> MPREIITLQLGQCGNQIGFEFWKQLCAEHGISPEGIVEEFATEGTDRKDVFFYQADDEHYIPRAVLLDLEPRVIHSILNSPYAKLYNPENIYLSEHGGGAGNNWASGFSQGEKIH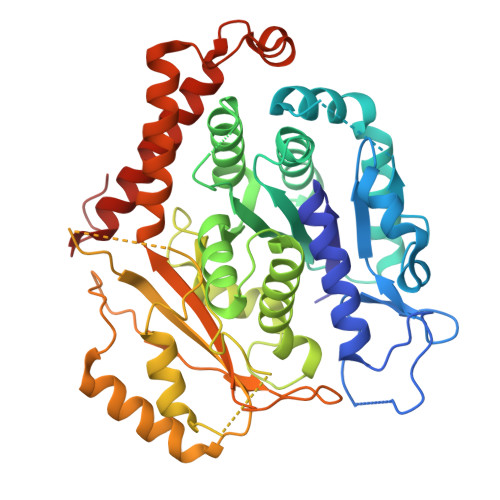EDIFDIIDREADGSDSLEGFVLCHSIAGGTGSGLGSYLLERLNDRYPKKLVQTYSVFPNQDEMSDVVVQPYNSLLTLKRLTQNADCVVVLDNTALNRIATDRLHIQNPSFSQINQLVSTIMSASTTTLRYPGYMNNDLIGLIASLIPTPRLHFLMTGYTPLTTDQSVASVRKTTVLDVMRRLLQPKNVMVSTGRDRQTNHCYIAILNIIQGEVDPTQVHKSLQRIRERKLANFIPWGPASIQVALSRKSPYLPSAHRVSGLMMANHTSISSLFERTCRQYDKLRKREAFLEQFRKEDMFKDNFDEMDTSREIVQQLIDEYHAATRPDYISWGTQEQ>[6x]MKHHHHHHQDEDEPSQSFESVALIIGVTGIVGNSLAEILPLSDTPGGPWKVYGVARRPRPTWNADHPIDYIQCDVSDAEDTRSKLSPLTDVTHVFYVTWTNRESESENCEANGSMLRNVLQAIIPYAPNLRHVCLQTGTKHYLGPFTNVDGPRHDP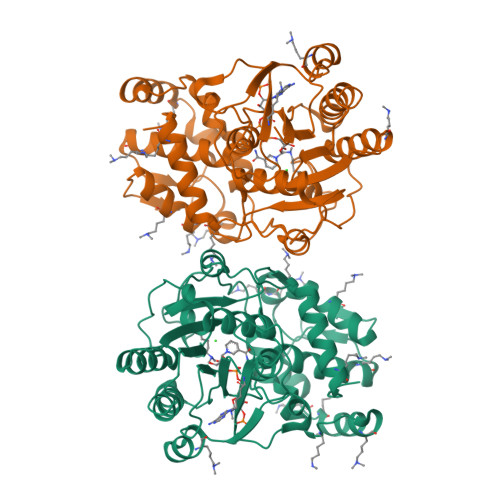PFTEDMPRLQIQNFYYTQEDILFEEIKKIETVTWSIHRPNMIFGFSPYSLMNIVGTLCVYAAICKHEGSPLLFPGSKKAWEGFMTASDADLIAEQQIWAAVDPYAKNEAFNCNNADIFKWKHLWKILAEQFGIEEYGFEEGKNLGLVEMMKGKERVWEEMVKENQLQEKKLEEVGVWWFADVILGVEGMIDSMNKSKEYGFLGFRNSNNSFISWIDKYKAFKIVP> MKCKFCSREAYIKIHYPKMYLCEEHFKEYFERKVSRTIERYKLLTKDERILVAVSGGKDSAVTAYVLKKLGYNIECLHINLGISGYSEKSEEYAKKQCKLIGAPLHIVRIKEILGYGIGEVKTRRPPCSYCGLTKRYIMNKFAYDNGFDAIATGHNLDDEASFLLNNILHWNTEYLAKGGPILPQQGKFIKKVKPLYEVTEREVVAYALAVGLEYIVEECPYARGATTLDMKGVLNELEEKRPGTKFNFVRGYLKKKKLFEPEIKEKEIKECKICRMPSSGDICAFCKFWGLKKEINFK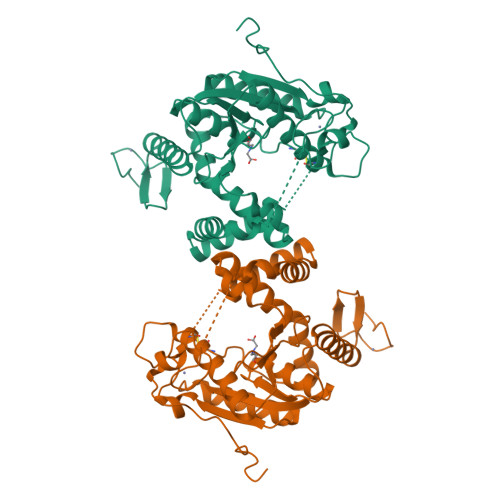VSSTDEEPFGP> TPWSKSELVRQLRDLGVRSGDMVMPHVSLRAVGPLADGPQTLVDALIEAVGPTGNILAFVSWRDSPYEQTLGHDAPPAAIAQSWPAFDPDH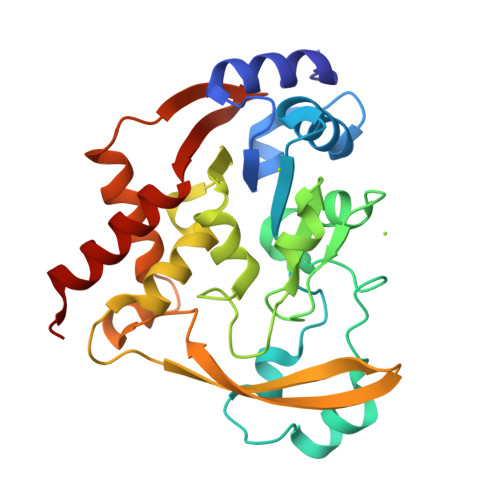APAYPGFGAINEFIRTYPGCRRSAHPDASMAAIGPDAAWLVAPHEMGAAYGPRSPIARFLAHAGKILSIGAGPDAVTALHYAEAVARIEGKRRVTYSMPLLREGKRVWVTTSDWDSNGILDEYAAPDGPDAVERIARDYLARTRVAQGPVGGAQSRLIDAADIVSFGIEWLEARHAA>RRKKGGWFGKHRGQGGSNPKFENIAEGLRALLARSHVERTTDEGTWVAGVFVYGG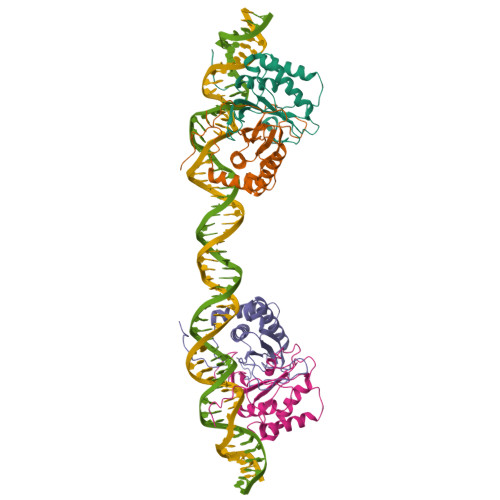SKTSLYNLRRGTALAIPQCRLTPLSRLPFGMAPGPGPQPGPLRESIVCYFMVFLQTHIFAEVLKDAIKDLVMTKPAPTCNIRVTVCSFDDGVDLPPWFPPMVEGA[4x]>[6x]ADVAGAVIDGAGLGFDVLKTVLEALGNVKRKIAVGIDNESGKTWTAMNTYFRSGTSDIVLPHKVAHGKALLYNGQKNRGPVATGVVGVIAYSMSDGNTLAVLFSVPYDYNWYSN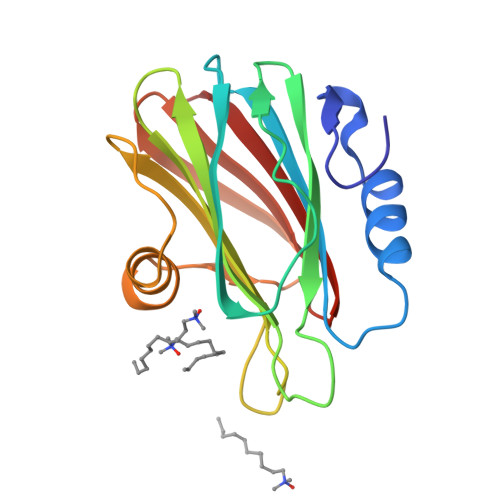WWNVRVYKGQKRADQRMYEELYYHRSPFRGDNGWHSRGLGYGLKSRGFMNSSGHAILEIHVTKA> MGSSHHHHHHSSGRENLYFQGMHALYITHPQVKIDPAVPVPEWGLSERGAERAREASRLPWAKALRRIVSSAETKAIETAHMLAETSGAAIEIIEAMHENDRSATGFLPPPEFEKAADWFFAHPEESFQGWERAIDAQARIVEAVKAVLDRHDARQPIA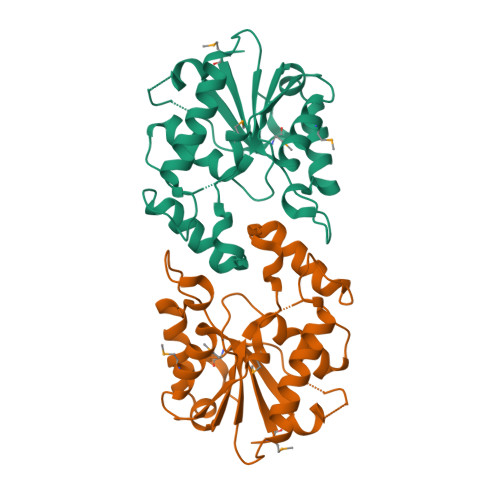FVGHGGVGTLLKCHIEGRGISRSKDQPAGGGNLFRFSIAEFSLAAASPTCDWTAMETWQG> KSAASSVGNAEDYAEETATSVKFKRSVTLPGCSSPLSLLGTGFREKKFAIIGVKVYAAGYYVNESILSGLSAWTGRSADEIQRDSSLFVSIFQAQAEKSLQIVLVRDVDGKTFWDALDEAISPRIKSPSSEDTTALSTFCCIFQNRPLNKGSVILLTWIN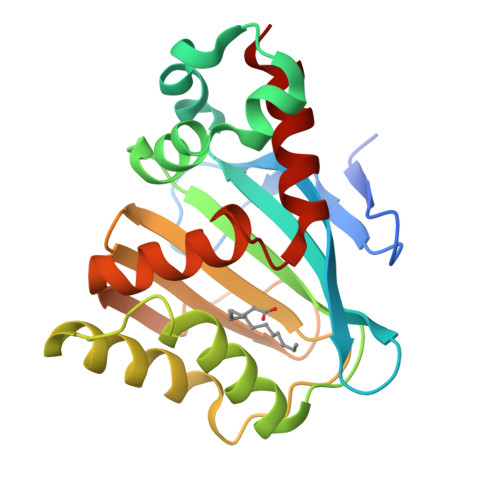TSNMLVSVSSGGLPTNVDATIESGNVTSALFDVFFGDSPVSPTLKSSVANQLAMTLV>[4x]GGSMKIKEVIV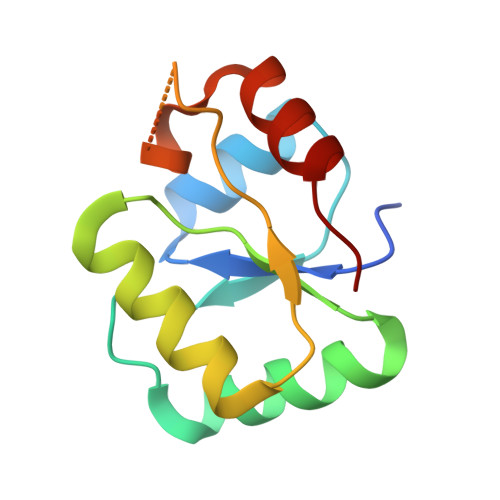VEGKDDTAAIRRAVDADTIETNGAAVGAEVIERIKLAKERRGVIIFTDPDFPGEKIRRTIAEQVPGCKHAFLPREAAKARSGKGIGVEHASPDDIRQALANVYEE>GTTSQKHRDFVAEPMGEKPVGSLAGIGEVLGKKLEERGFDKAYVVLGQFLVLKKDEDLFREWLKDTAGANAKQS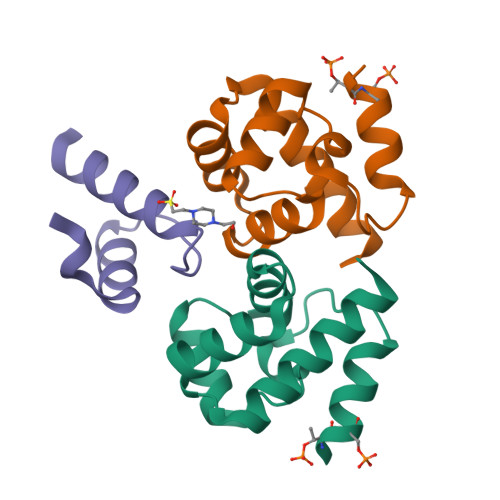RDAFGALREWADAFL[2x];> GDNYADLSDTELTTLLRRYNIPHGPVVGSTRRLYEKKIFEYETQRRRLSPPSSSAASSYSFSDLNSTRGDADMYDLPKKEDALLYQSKGYNDDYYEESYFTTRTYGEPESAGPSRAVRQSVTSFPDADAFHHQVHDDDLLSSSEEECKDRERPMYGRDSAYQSITHYRPVSASRSSLDLSYYPTSSS> MSQSNRELVVDFLSYKLSQKGYSWSQPMAAVKQALREAG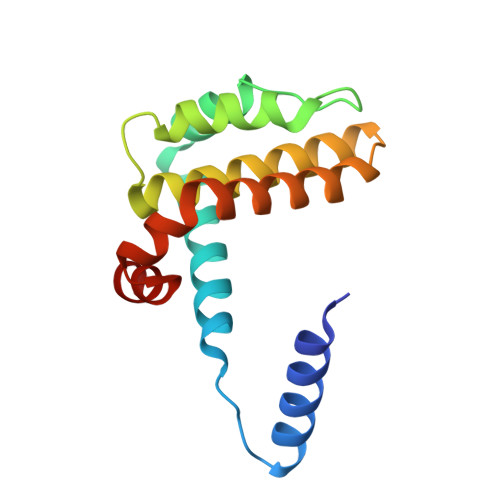DEFELRYRRAFSDLTSQLHITPGTAYQSFEQVVNELFRDGVNWGRIVAFFSFGGALCVESVDKEMQVLVSRIAAWMATYLNDHLEPWIQENGGWDTFVELYG>[2x]MDRRFPPFSPFFNHGRFFDDVDFDRHMIRPYWADQTMLTGHRVGDAIDVVNNDQEYNVSVDVSQFEPEELKVNIVDNQLIIEGKHNEKTDKYGQVERHFVRKYNLPTGVRPEQIKSELSNNGVLTVKYEKNQEQQPKSIPITIVPKRN

Small Heat shock proteins (sHsps) are a family of molecular chaperones that bind nonnative proteins in an ATP-independent manner. Caenorhabditis elegans encodes 16 different sHsps, among them Hsp17, which is evolutionarily distinct from other sHsps in the nematode. The primary structure of sHsps shows a conserved organization with three functional segments: the α-crystallin domain (ACD) which is surrounded by the highly flexible N-terminal region (NTR) and a short C-terminal region (CTR). Consistent with its presence under nonstress conditions, and in contrast to many other sHsps, we determined that Hsp17 is a mono-disperse, permanently active chaperone in vitro, which interacts with hundreds of different C. elegans proteins under physiological conditions.

To address the basis for the special chaperone mechanism of Hsp17, we solved the structure of the Hsp17 wt 24-mer by cryo-EM. The oligomer has a cubic shape with the symmetry of a regular tetrahedron. The edges of the cube are represented by ACD dimers resulting in a 24-mer structure. In line with findings on other sHsps, the overall resolution of the EM reconstitution is 6.49 Å with the different parts of Hsp17 differing in resolution. Thus, in contrast to previous results, our reconstruction shows that Hsp17 adopts the metazoan ACD dimer interface. The NTRs of the surface-facing monomers are oriented to the outside of the oligomer and are partly unresolved, whereas the NTRs of the inward-facing monomers protrude towards the inside of the oligomer and interact with each other. In both types, the link between the monomers is established by the binding of the I-x-I motif of the CTR into the pocket formed by the β4 and β8 strands of the ACD of a neighboring monomer. We were able to generate a pseudo-atomic model of the Hsp17 24-mer consisting of residues 25 to 148 for the surface monomer and residues 1 to 148 for the inward-facing monomer. Hsp17’s unique trait is based on the specific arrangement of the NTRs which functionally separates them into two groups: those involved in formation and stabilization of the 24-mer in the inside of the cube and those accessible for substrate on its outside.> MEEYQVKIDTFEGPLDLLLHLINRLEIDIYDIPVAKITEQYLLYVHTMRVLELDIASEYLVMAATLLS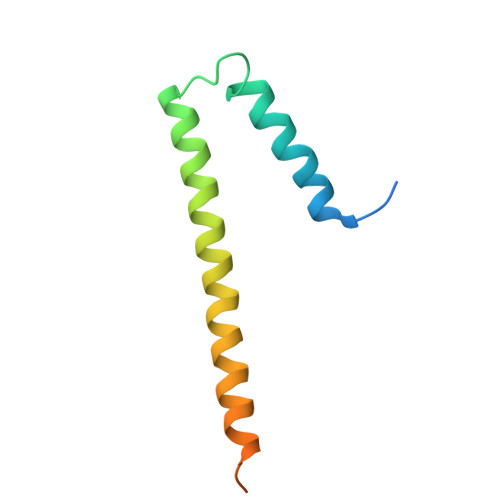IKSRMLLPKQEEELFEDETSHHHHHH> MGNVQTSVNTYNITGDGNSFTPTSDMTSTAAPAID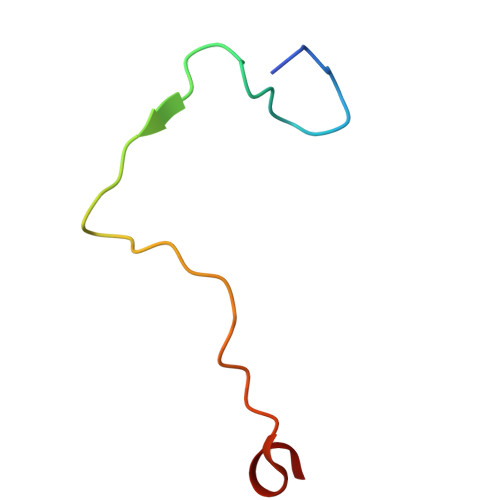LKPGVLN>[3x]MRGSAFNGKWETESQEGYEPFCKLIGIPDDVIAKGRDFKLVTEIVQNGD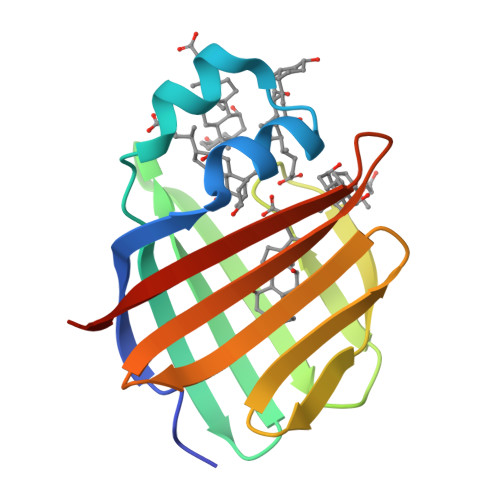DFTWTQYYPNNHVVTNKFIVGKESDMETVGGKKFKGIVSMEGGKLTISFPKYQQTTEISGGKLVETSTASGAQGTAVLVRTSKKVLVPR Phytochromes are red-light photoreceptors found in various plants and microorganisms. S. aurantiaca contains two previously uncharacterized bacteriophytochromes (BphPs) denoted SaBphP1 and SaBphP2, which may be responsible for the light-stimulated growth of multicellular fruiting bodies. The classical BphPs switch between a red absorbing state denoted Pr (λmax ≃ 700 nm) and a far-red absorbing state denoted Pfr (λmax ≃ 750 nm).

The SaBphP1 and other myxobacterial BphPs lack a conserved histidine (His) at position 289 in the GAF domain. SaBphP1 contains a threonine (Thr289) at this position, which is replaced by glycine in some myxobacterial BphPs. The mutant PCM also crystallizes in the dark in the Pr state in P3221 with three subunits denoted A, B and C in the asymmetric unit, but the PCM-wt crystallized in space group C2 with a single, dimeric BphP molecule in the asymmetric unit. Interestingly, the crystallization conditions for the PCM wild-type and T289H mutant are the same, yet they crystallize in different space groups. Indeed, the r.m.s.d. between the T289H mutant and wild-type PCM is ∼3 Å overall. As shown in Fig. 5(b) and Table 2, the PAS and GAF domains superimpose well, but the PHY domains occupy different positions. When this His is absent, as in the SaBphP1-PCM-wt, the formation and stabilization of the Pfr state is impeded. The resolution achieved with wild-type SaBphP1-PCM (2.25 Å) is the highest so far reached for unmodified PCM dimers. Hence, the SaBphP1-PCM crystals are perfectly suited to reach the near atomic resolution range (∼2.5 Å) in TR-SFX experiments.

>[2x]MSTEASRSGKQEVDLTNCDREPIHIPGAIQPHGVLLVLSEPGLVLTHASENAPAVLGNSAEQLLGAPLGHFIEPSVREPLEADLRSARLKQLNPLKVVWRVDGVDRFFDGIAHRHQGRLILELEPSSHREAVPFLSFFHAVRDGLSRLRDARDLQELCEAVVQEVRGLTGFDRAIIYRFDAEWNGSVIAEARDARADPYLGLHFPASDIPRQARELYQLNWLRIIPTIDYQPARVRALPGHGEPLDLSFSVLRSVSPIHLEYLHNMGVQASMSISLMKDGKLWGLISCTQVSGTRYVPYEVRTACEFLGEVMSSLLAAKEGNEDYDQRIRAKSIHAALLERMAREVDFVSGLASQESGLLELVHAHGAAIHFHGRTTVLGQAPSDEALTGLIEWLGSRTGEGVFCTDRLAREYPEAQAFQEVAAGLMAFSMSRGRNNFVLWFRPEAVQTVNWSGNPTKAVEFDQGGPRLHPRKSFELWKETVRGRCLPWKAYEVEAASELRRSIIDVALQRSE> GAHMGDFLASLEQDIKPAFGTNQEDYASYIMNGIIKWGDPVTRVLDDGELLVQQTKNSDRTPLVSVLLEGPPHSGKTALAAKIAEESNFPFIKICSPDKMI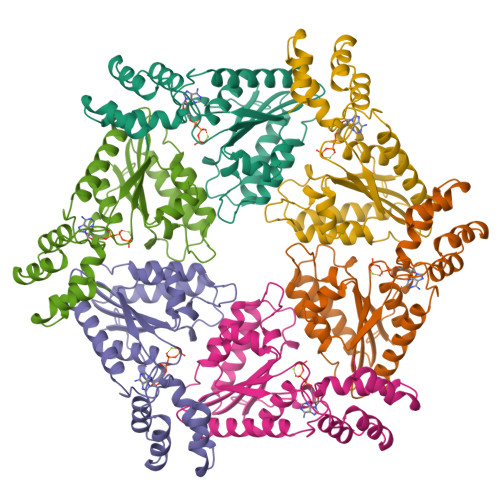GFSETAKCQAMKKIFDDAYKSQLSCVVVDDIERLLDYVPIGPRFSNLVLQALLVLLKKAPPQGRKLLIIGTTSRKDVLQEMEMLNAFSTTIHVPNIATGEQLLEALELLGNFKDKERTTIAQQVKGKKVWIGIKKLLMLIEMSLQMDPEYRVRKFLALLREEGASPLDFDLE>[2x]XPLVVAASII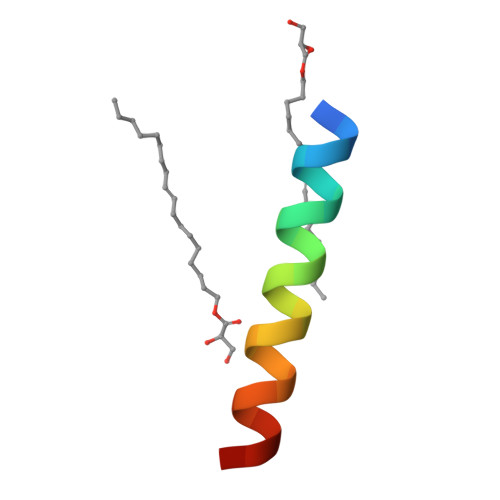AILHLILWILDRLX>GSMAVTNVAELNALVERVKKAQREYASFTQEQVDKIFRAAALAAADARIPLAKMAVAESGMGIVEDKVIKNHFASEYIYNAYKDEKTCGVLSEDDTFGTITIAEPIGIICGIVPTTNPTSTAIFKSLISLKTRNAIIFSPHPRAKDATNKAADIVLQAAIAAGAPKDLIGWIDQPSVELSNALMHHPDINLILATGGPGMVKAAYSSGKPAIGVGAGNTPVVIDETADIKRAVASVLMSKTFDNGVICASEQSVVVVDSVYDAVRERFATHGGYLLQGKELKAVQDVILKNGALNAAIVGQPAYKIAELAGFSVPENTKILIGEVTVVDESEPFAHEKLSPTLAMYRAKDFEDAVEKAEKLVAMGGIGHTSCLYTDQDNQPARVSYFGQKMKTARILINTPASQGGIGDLYNFKLAPSLTLGCGSWGGNSISENVGPKHLINKKTVAKRAENMLWHKLPKSIYFRRGSLPIALDEVITDGHKRALIVTDRFLFNNGYADQITSVLKAAGVETEVFFEVEADPTLSIVRKGAELANSFKPDVIIALGGGSPMDAAKIMWVMYEHPETHFEELALRFMDIRKRIYKFPKMGVKAKMIAVTTTSGTGSEVTPFAVVTDDATGQKYPLADYALTPDMAIVDANLVMDMPKSLCAFGGLDAVTHAMEAYVSVLASEFSDGQALQALKLLKEYLPASYHEGSKNPVARERVHSAATIAGIAFANAFLGVCHSMAHKLGSQFHIPHGLANALLICNVIRYNANDNPTKQTAFSQYDRPQARRRYAEIADHLGLSAPGDRTAAKIEKLLAWLETLKAELGIPKSIREAGVQEADFLANVDKLSEDAFDDQCTGANPRYPLISELKQILLDTYYGRDYVEGETAAKKEAAPAKAEKKAKKSA[8x]

Aldehyde-alcohol dehydrogenase (AdhE) is a bifunctional aldehyde-alcohol dehydrogenase highly conserved in bacteria as well as fungus, algae, and protozoan parasites. The N-terminal aldehyde dehydrogenase (ALDH) domain converts acetyl-CoA to acetaldehyde, which is then converted to ethanol by the C-terminal alcohol dehydrogenase (ADH) domain. Structurally, AdhE is interesting as this 96 kDa protein oligomerises to form long filaments which can be visualised by electron microscopy. Here, we present an atomic resolution cryo-EM structure of AdhE forming a spirosome and show that this spirosome formation is critical for AdhE activity.

160,830 particles out of 251,604 particles picked were further processed using cisTEM 14 to generate a 3.5 Å resolution cryo-EM map. Most of the side chains were resolved in the cryo-EM map, and we built atomic models of six complete AdhE molecules and two ADH domains. These molecules are stacked upon each other to form a right-handed helix with a 70 Å helical pitch and 150 Å diameter. The cryo-EM structure of AdhE shows that the ALDH and ADH domains in the AdhE monomer are separated by a linker (residues 441–448). Together with a β-hairpin protruding from the ALDH domain, the linker makes a three-stranded β-sheet stabilizing connections between the two catalytic domains. Two AdhE monomers form a dimer in a head-to-head arm-crossing fashion. Subsequently, two dimers (four AdhE molecules) form one helical pitch via the interaction of ADH domains in a tail-to-tail manner. F670 in the ADH domain is inserted into a hydrophobic pocket formed by F462, I460, and I712 of the other ADH domain and holds the ADH-ADH domains together. To further investigate the implication of the spirosome structure of AdhE, the plausible active sites of ALDH and ADH were highlighted on the helical structure. This practice reveals that ALDH active sites are located towards the outer surface of the helical structure while ADH active sites reside towards the inner surface. Compared with WT, a dramatic decrease in the AdhE activity was observed for the mutants defective in spirosome formation, implying that the spirosome formation that we observed in the cryo-EM structure is important for AdhE activity.>MFLEAVYHRPRKNF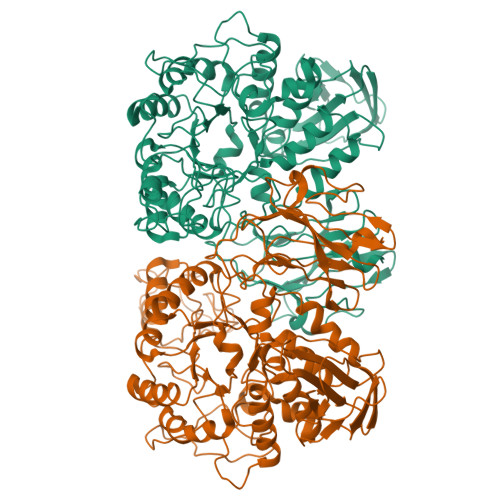SYAYNGTTVHLRIRTKKDDMTAVYALAGDKYMWDHTMEYVPMTKLATDELFDYWECEVTPPYRRVKYGFLLQQGHEKRWMTEYDFLTEPPANPDRLFEYPFINPVDVFQPPAWVKDAIFYQIFPERFANGDTRNDPEGTLPWGSADPTPSCFFGGDLQGVIDHLDHLSKLGVNAVYFTPLFKATTNHKYDTEDYFQIDPQFGDKDTLKKLVDLCHERGIRVLLDAVFNHSGRTFPPFVDVLKNGEKSKYKDWFHIRSLPLEVVDGIPTYDTFAFEPLMPKLNTEHPDVKEYLLKAAEYWIRETGIDGWRLDVANEVSHQFWREFRRVVKQANPDAYILGEVWHESSIWLEGDQFDAVMNYPFTNAVLDFFIHQIADAEKFSFMLGKQLAGYPRQASEVMFNLLDSHDTARLLTQADGDKRKMKLAVLFQFTYFGTPCIYYGDEVGLDGGHDPGCRKCMEWDETKHDKDLFAFYQTVIRLRQAHAALRTGTFKFLTAEKNSRQIAYLREDDQDTILVVMNNDKAGHTLTLPVRHAQWTHLWQDDVLTAAHGQLTVKLPAYGFAVLKASSD[2x]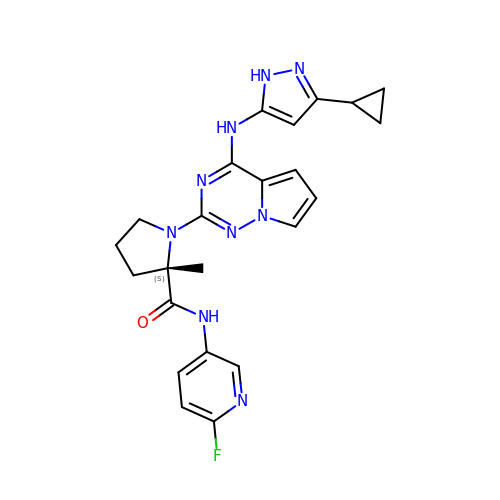1-{4-[(3-cyclopropyl-1H-pyrazol-5-yl)amino]pyrrolo[2,1-f][1,2,4]triazin-2-yl}-N-(6-fluoropyridin-3-yl)-2-methyl-L-prolinamide | C23 H24 F N9 O | LQVXSNNAFNGRAH-QHCPKHFHSA-N>[2x]GSHMSFSGKYQLQSQENFEAFMKAIGL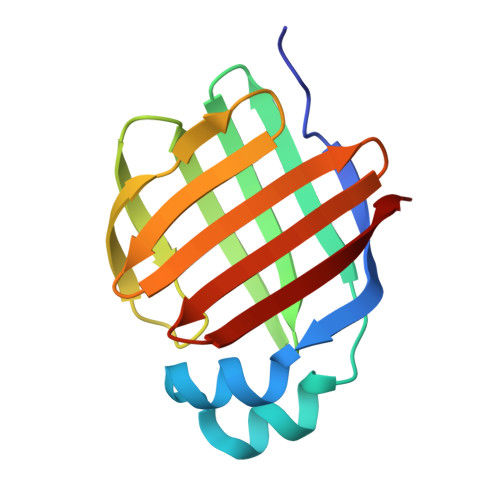PEELIQKGKDIKGVSEIVQNGKHFKFTITAGSKVIQNEFTVGEECELETMTGEKVKTVVQLEGDNKLVTTFKNIKSVTELNGDIITNTMTLGDIVFKRISKRI> MRGSHHH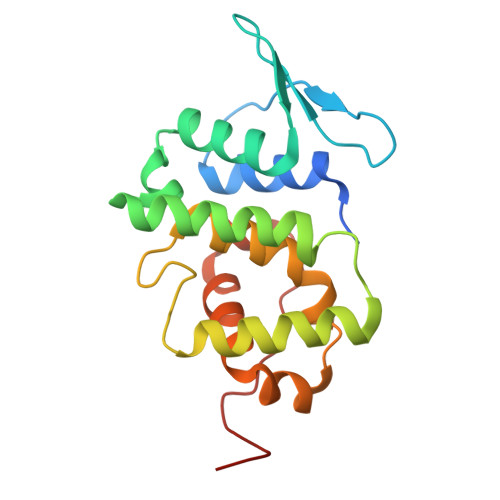HHHGSMAAAAELSLLEKSLGLSKGNKYSAQGERQIPVLQTNNGPSLTGLTTIAAHLVKQANKEYLLGSTAEEKAIVQQWLEYRVTQVDGHSSKNDIHTLLKDLNSYLEDKVYLTGYNFTLADILLYYGLHRFIVDLTVQEKEKYLNVSRWFSHIQHYPGIRQHLSSVVFIKNRLYTNSH>AAASMSALITENMHMKLYMEGTVNNHHFKCTSEGEGKPYEGTQTMRIKVVEGGPLPFAFDILATSFMYGSKTFINHTQGIPDFFKQSFPEGFTWERVTTYEDGGVLTATQDTSLQDGCLIYNVKIRGVNFPSNGPVMQKKTLGWEACTEMLYPADGGLEGRSDMALKLVGGGHLICNLKTTYRSKKPAKNLKMPGVYYVDRRLERIKEADKETYVEQHEVAVARYCDLP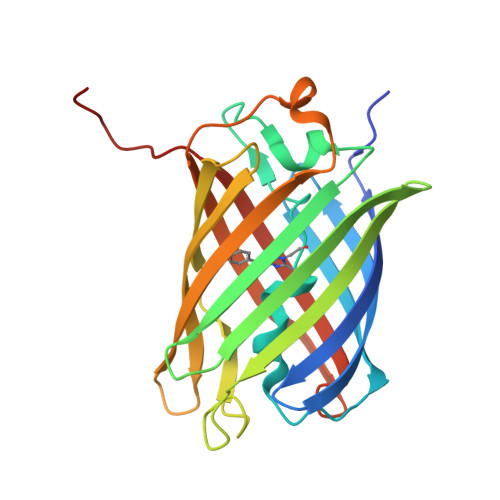SKLAHK[4x]> NAWDRTL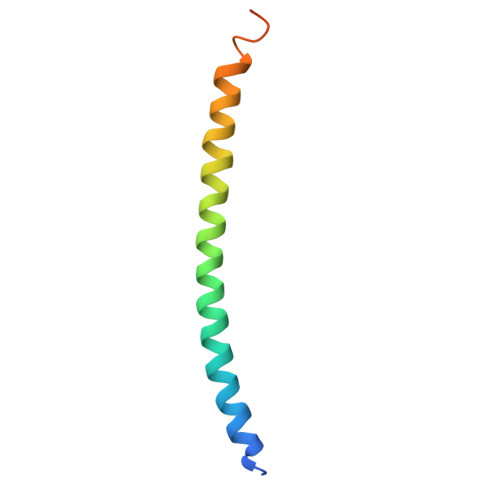IENGEKITSLHREVEKVKLDQKRLDQELDFILSQQKELEDLLSPLEESVKEQSGTIY> MAEAGEILIKGGKVVNEDCSFFSDVHIRGGKIVEVGP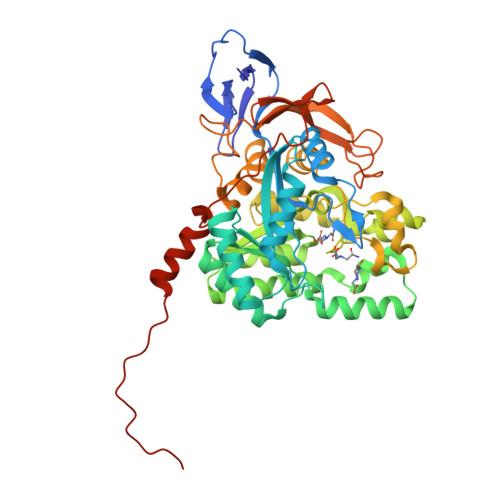DLRVPPGARVIDATDRLVIPGGIDTHTHMELAFMGTRAVDDFHIGTKAALAGGTTMILDFVMTQKGQSLLEAYDLWRKTADPKVCCDYSLHVAVTWWSDEVKDEMRTLAQERGVNSFKMFMAYKGLFMLRDDELYAVFSHCKEVGAIAQVHAENGDLIAEGAKKMLSLGITGPEGHELCRPEAVEAEATQRAITIASAVNCPLYVVHVMSKSAADVVSKARKDGRVVFGEPIAASLGTDGTNYWHKDWAHAAQYVMGPPLRPDPSTPGYLMDLLANDDLTLTGTDNCTFSRCQKALGKDDFTRIPNGVNGVEDRMSVIWEKGVHSGKMDENRFVAVTSSNAAKIFNFYPQKGRIAKDSDADVVIWDPKTTRKISAQTHHQAVDYNIFEGMECHGVPVVTVSRGRVVYEEGRLKVSPGQGRFIHRQPFSEFVYKRIRQRDEVGKPAVVIREPYAGEVVALGTSD> VDATFYTSDEALEAATAPLYNRAWFDYNQRSIVPIGSGRANDMYSPWNYPQFVTFQVTALDENLSGAWSGFYSVVTMANSVINAVETQTQGSVSEAAKTKAIAEARLMRACAYFYMLRIWGPVILIEDNQKLVDNPVRPLNREEDVFQFIINDLNYAVDNLSEQSDKGRATSWAAKGILAKVYLARSGWNNGGTRDEGDLELARQYASDVCENSGLDLMTNYEDLFKYKNNNNQESLLAMQWVPLGEWYECNTLLSDLAFSTEVTGGVNCWSSYNGSIDMLQQYELADTLRRNATFFTKGSYYSYICIKDGGYTYKGTASPIKKGVPGGPDDDNDGKVKQMNSPLNTYILRLADVYLTYAEACLGNNSTLSDGRGL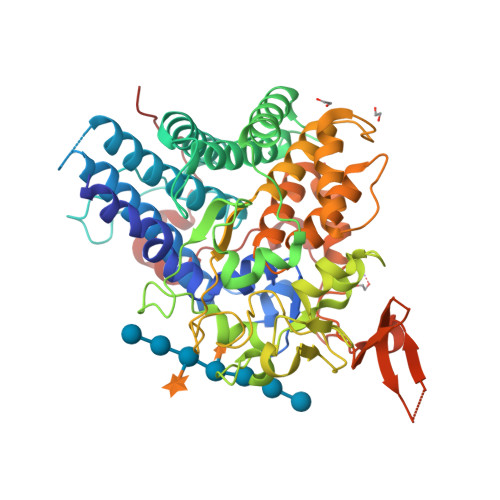YFFNRVRERAKINKKSSITLDDIIRERRVEFGMEYSNWYDMVTWFRYLPDKMLNYFNNQWRGYRTDAIIKDEDGKLHFGKYDTDGTTFLEGPEYYTAPEFTINIEAEDIFLPYPESDVIQNPLLNEPPVPYTFNE> SNADDLREPEERHLDDAFF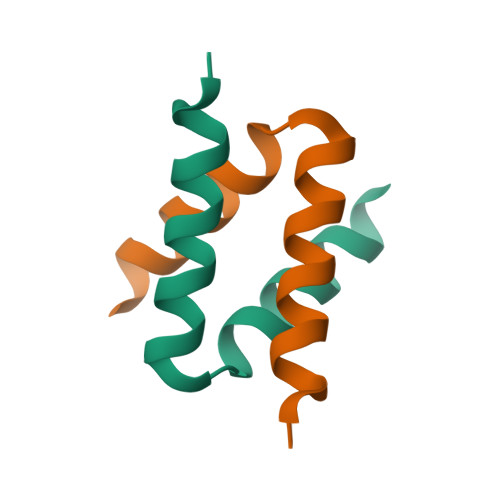RGYKNLEPEAKAQLRKMLDTFKKDF>[15x]TTSSQKFIARNRAPRVQIEYDVELYGA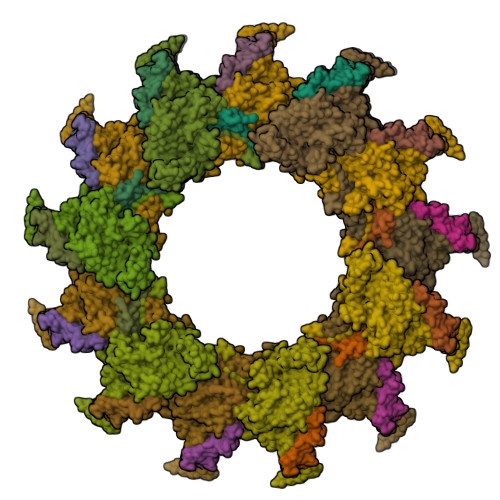EKKVQLPFVMGVMADLAGKPAEPQAAVADRKFLEIDVDNFDARLKAMKPRVAFNVPNVLTGEGNLSLDITFESMDDFSPAAVARKVDSLNKLLEARTQLANLLTY;>REAVETAVRTLAEHALEQTSLISNDAIKSIESIIAALDAKLTAQVNLIMHHADFQQLESAWRGLHYLVNNTETDEQLKIRVLNISKPELHKTLKKFKGTTWDQSPIFKKLYEEEYGQFGGEPYGCLVGDYYFDQSPPDVELLGEMAKISAAMHAPFISAASPTVMGMGSWQELSNPRDLTKIFTTPEYAGWRSLRESEDSRYIGLTMPRFLARLPYGAKTDPVEEFAFEEETDGADSSKYAWANSAYAMAVNINRSFKLYGWCSRIRGVESGGEVQGLPAHTFPTDDGGVDMKCPTEIAISDRREAELAKNGFMPLLHKKNTDFAAFIGAQSLQKPAEYDDPDATANANLAARLPYLFATCRFAHYLKCIVRDKIGSFKEKDEMQRWLQDWILNYVDGDPAHSTETTKAQHPLAAAEVVVEEVEGNPGYYNSKFFLRPHYQLEGLTVSLRLVSKLPSAKEA[15x]>GGKKFILELIETVYEEILDLEANLRNGQQTDSTAMWEALHIDDSSYDVNPFISMLSFDKGIKIMPRIFNFLDKQQKLKILQKIFNELSHLQIIILSSYKTTPKPTLTQLKKVDLFQMIILKIIVSFLSNNSNFIEIMGLLLQLIRNNNVSFLTTSKIGLNLITILISRAALIKQDSSRSNILSSPEISTWNEIYDKLFTSLESKIQLIFPPREYNDHIMRLQNDKFMDEAYIWQFLASLALSGKLNHQRIIIDEVRDEIFATINEAETLQKKEKELSVLPQRSQELDTELKSIIYNKEKLYQDLNLFLNVMGLVYRDGEISELKHHHHHH[2x]

The Pat1 protein is involved in different aspects of mRNA decapping activation. Hence, Pat1 is considered as a central platform protein for decapping. Indeed, the crystal structure of the S. cerevisiae Pat1C shows that this domain structurally belongs to the ARM repeat superfamily, which mostly encompasses proteins involved in protein-protein interaction. In conclusion, the crystal structure of the ScPat1 C-terminal domain has revealed two functionally important regions localized at opposite extremities of the domain.

We therefore cloned the ScPat1C (473-796) domain, over-expressed it in E. coli and purified it in milligram amounts to homogeneity. The SeMet labeled and unlabeled proteins crystallized in three different space groups. Only structures refined to higher resolution (crystal forms II and III) will be discussed in this manuscript. Three and two copies of the ScPat1C molecule are present in the asymmetric unit of crystal forms II and III, respectively. The crystal packing radically differs between crystal forms II and III. In crystal form III, the two Pat1 molecules of the asymmetric unit exhibit a very intricate head-to-tail organization with an interacting surface area of 1,635 Å2. As this value is in the range expected for interfaces within homodimers, this suggested that this ScPat1C domain could also exist as a homodimer in solution. To investigate this possibility, we have analysed the quaternary structure of ScPat1C in solution using both size exclusion chromatography coupled online to a triple detection array (MALLS) and small angle X-ray Scattering (SAXS). MALLS measurements on a protein at 2 mg/mL yielded a molecular mass of 39.3 kDa, indicating that ScPat1C is monomeric in solution (the theoretical molecular weight for the monomer is 38.6 kDa). Furthermore, the SAXS experimental curves measured at various ScPat1C concentrations (5.4 and 11.2 mg/mL, i.e. concentrations closer to those used in the crystallization experiments) clearly correspond to the curve calculated from the coordinates of the ScPat1C monomer but not from those of the crystal dimer. This SAXS analysis indicates that: first, the large contact area observed in crystal form III is created by the crystal-packing and does not reflect a biologically relevant oligomeric state; second, ScPat1C adopts in solution a structure similar to that observed in the crystals.Type 2 promoters contain two gene-internal DNA-binding elements named A- and B-box that are recognized by the general transcription factor IIIC (TFIIIC). TFIIIC is a six-subunit protein complex of ∼0.5 MDa mass consisting of two subcomplexes of similar size, τA and τB, which contact A-box and B-box promoter elements, respectively. We therefore structurally characterized the S. pombe TFIIIC Sfc1/Sfc7 subcomplex and present crystal structures of two structural modules. The N-terminal moiety of Sfc1 (Sfc1-NT) and subunit Sfc7 heterodimerize through a triple β-barrel fold most similar to the dimerization domains of general transcription factor TFIIF Rap30/Rap74, whereas the C-terminal DNA-binding domain of Sfc1 (Sfc1-DBD) comprises a winged-helix domain most similar to the winged-helix domain present in TFIIF Rap30 that is packed against a second domain with novel fold.

Well-diffracting crystals were obtained for a Sfc11-110(K48A,Q49A)/Sfc71-101 construct, where two non-conserved Sfc1 residues (K48 and Q49) were mutated into alanine following the suggestion of the surface entropy reduction prediction (SERp) server. The structure was solved at 2.4 Å by single-wavelength anomalous diffraction using para-chloro-mercuribenzene sulfonate as heavy-atom derivate. The Sfc1-NT/Sfc7 dimerization module consists of three interwoven β-barrels containing 15 β-strands and four α-helices. The interwoven structure suggests that the subunits fold co-operatively and need to be simultaneously expressed. The crystal structure also confirmed that the mutated residues K48 and Q49 lay at the surface of the Sfc1 dimerization domain and do not interfere with Sfc1–Sfc7 heterodimerization. According to program Dali, the structure shares the highest similarity with the TFIIF Rap30/Rap74 dimerization domains. Sfc1 and Sfc7 resemble Rap30 and Rap74, respectively (Z-score = 9.3, rmsd154CA = 4.7 Å). Despite the readily apparent structural similarity between Sfc1 and Rap30 and Sfc7 and Rap74, Sfc1 helices α1 to α3 and β-strands β3 and β4 replace Rap30 strands β3 and β4 (approximately residues 20–68), whereas the ‘arm domain’ of Rap74 is absent in Sfc7. The Sfc1-NT/Sfc7 dimerization domain can also be superimposed with the dimerization modules of Pol I subunits A49/A34.5 (Z-score = 7.7, rmsd142CA = 4.2 Å) and mouse RNase H2B/H2C (Z-score = 7.8, rmsd134CA = 3.7 Å).

> GAMGSLKISDNEYALIEHPGFANNKDAFFQTLGGVQSIQKACQTSFQNPAAALLELNLRPKDKYHHPVQARVQSRNDLLVTIKKMDNSVQNVSRIRQVFLFRDMADFQYSTQ;> SSNSPSLETDVDDVENIVFQFQNSSLDFQSSDDFSILGIDQPHPIVRIGGMFFRGTWHQPIGTDIVVPSVNDSELSRDGLVLCKRRLMLEQIRLVPKNPS Phosphorylated arginine residues (pArg) serve as a degradation signal that is recognized by the ClpC:ClpP (ClpCP) protease, a quasi-proteasomal particle critical for microbial protein quality control, stress tolerance, and pathogenicity (Trentini et al., 2016). ClpC carries out its quality control function by acting as an ATP-driven unfoldase that selects certain client proteins and translocates them into the protease compartment formed by ClpP. The ClpC protomer contains an amino-terminal domain (ClpCNTD), two AAA (ATPases associated with diverse cellular activities) domains termed D1 and D2, and a coiled coil (M domain) inserted into D1. In the active ClpC hexamer, the D1 and D2 domains form two stacked ATPase rings that power substrate unfolding and translocation.

To stabilize ATP-mediated contacts between ClpC protomers, we used a catalytically inactive mutant (E280A/E618A, referred to as ClpCDWB) that binds ATP but does not hydrolyze it. To resolve the functional units of the activated unfoldase at higher resolution, we performed a focused cryo-EM analysis of the single hexamers. The resulting 3D map had an overall resolution of 3.7 Å and allowed us to build an atomic model of the substrate-bound ClpC complex. The most prominent feature of the cryo-EM reconstruction is a well-defined, 80-Å-long density that penetrates the entire ClpC pore, proceeding from the top of the D1 to the bottom of the D2 ring. Although it is not possible to discern side chains, the density should represent the protein backbone of the captured mSA-Kre substrate, comprising 26 residues present in an extended conformation. The six ClpC subunits adopt a spiral arrangement, engaging the substrate in a similar manner to that observed in the related double-ring AAA unfoldases ClpA, ClpB, and Hsp104 (Gates et al., 2017; Lopez et al., 2020; Rizo et al., 2019). Five ClpC protomers (P1–P5, P1 as lowermost and P5 uppermost unit in the AAA ring) interact with the substrate through conserved tyrosine-bearing pore loops in the D1 and D2 domains, while the “seam” protomer (P6) is detached from the substrate, transitioning from the bottom to the top position of the spiral. In both rings, the substrate-engaging P2–P5 protomers are present in an ATP-bound state (except P2-D2), whereas protomers P1 and P6 accommodate ADP or are present in an apo state. These structural data are consistent with the previously suggested “hand-over-hand” translocation mechanism (Puchades et al., 2020), according to which nucleotide exchange is coupled with substrate release and upward movement of the seam protomer P6 to rebind ATP and substrate. In conclusion, the cryo-EM structure of the reconstituted ternary complex provides a snapshot of ClpC in the process of unfolding a BacPROTAC-tethered substrate.

>MMFGRFTERAQKVLALAQEEALRLGHNNIGTEHILLGLVREGEGIAAKALQALGLGSEKIQKEVESLIGRGQEMSQTIHYTPRAKKVIELSMDEARKLGHSYVGTEHILLGLIREGEGVAARVLNNLGVSLNKARQQVLQLLGSNETGSSAAGTNSNANTPTLDSLARDLTAIAKEDSLDPVIGRSKEIQRVIEVLSRRTKNNPVLIGEPGVGKTAIAEGLAQQIINNEVPEILRDKRVMTLDMGTVVAGTKYRGEFEDRLKKVMDEIRQAGNIILFIDALHTLIGAGGAEGAIDASNILKPSLARGELQCIGATTLDEYRKYIEKDAALERRFQPIQVDQPSVDESIQILQGLRDRYEAHHRVSITDDAIEAAVKLSDRYISDRFLPDKAIDLIDEAGSKVRLRSFTTPPNLKELEQKLDEVRKEKDAAVQSQEFEKAASLRDTEQRLREQVEDTKKSWKEKQGQENSEVTVDDIAMVVSSWTGVPVSKIAQTETDKLLNMENILHSRVIGQDEAVVAVAKAVRRARAGLKDPKRPIGSFIFLGPTGVGKTELARALAESIFGDEESMIRIDMSEYMEKHSTSRLVGSPPGYVGYDEGGQLTEKVRRKPYSVVLLDAIEKAHPDVFNILLQVLEDGRLTDSKGRTVDFRNTILIMTSNVGASELKRNKYVGFNVQDETQNHKDMKDKVMGELKRAFRPEFINRIDEIIVFHSLEKKHLTEIVSLMSDQLTKRLKEQDLSIELTDAAKAKVAEEGVDLEYGARPLRRAIQKHVEDRLSEELLRGNIHKGQHIVLDVEDGEFVVKTTAKTNLEHHHHHH[6x]> MSGSMEKLAEIMQEIIEAYQEVKDAFFKFIKAVHEGAPEEELKKYLEKMKEALEKMKELLERLEKEAKKVIEENKDKKLELKVLLMLRLAYLLLKVSIELTKIAAEKLGDKELVEELEKESKEVEKKIKELEE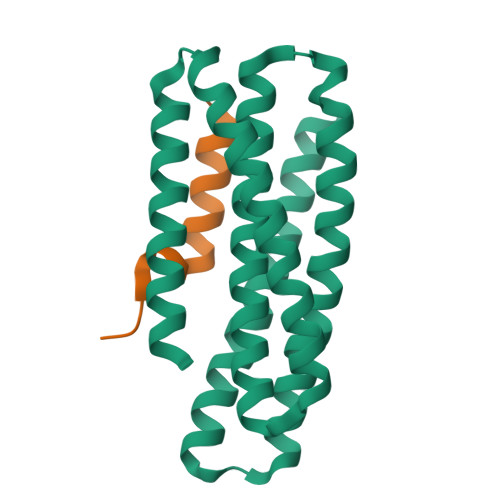RIKKLLEEVDDEELKEAYKEVEEMEKEAEKFLEKMRKVGSG;> HSQGTFTSDYSKYLDSRRAQDFVQWLMNT>ATQGVFTLPANTQFGVTAFANSAGTQTVNVQVNNETVATFTGQSTNNAIIGSKVLNSGGGGKVQILVSVNGRSSDLVSAQVILANELNFALVGSEDSTD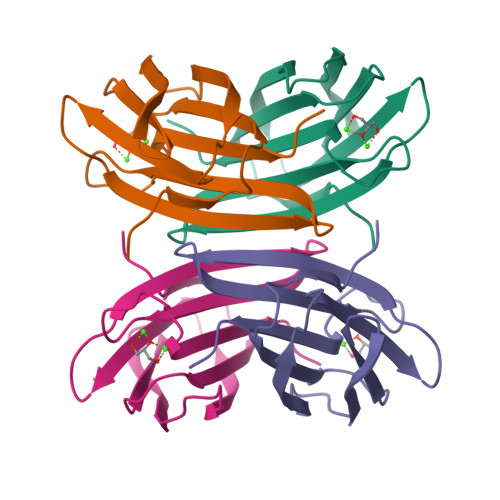NDYNDAVVVINWPLG[4x]Given the auxotrophic nature of pneumococci for certain amino acids, the Ami ABC transporter system, orchestrating oligopeptide uptake, becomes indispensable in host compartments lacking amino acids. The system comprises five exposed Oligopeptide Binding Proteins (OBPs) and four proteins building the ABC transporter channel. Crucially, SBPs determine the specificity of their respective transport systems, thereby governing the range of molecules capable of entering the cell. The five lipoproteins exhibit pairwise sequence identity of ~52–60% and share a very similar overall folding.

Consequently, the 1.8 Å-resolution open conformation of AliD was selected as a representative structure to describe the global architecture of OBPs in the Ami system. The obtained electron density map of the AliD structure, encompassing residues 28 to 652, presents an excellent quality all over the sequence. AliD adopts a bilobate structure characterized by three domains interconnected by short polypeptide chain segments serving as hinges. The two lobes enclose a deep cavity measuring ~16 Å in width and 45 Å in height, housing the peptide-binding pocket. Lobe 1 comprises Domain I (residues 29–63, 191–296, and 583–617) and Domain II (residues 64–190), while Lobe 2 consists solely Domain III (residues 297–582). The most striking feature of the AliD structure compared to OppA is the presence of an intriguing additional C-terminal 30-aa long α-helix (α19, spanning residues 622–652). This α-helix, which serves as distinctive hallmark of all the Ali proteins, establishes numerous hydrophobic and polar interactions with Domains I and II from Lobe 1, contributing significantly to the structural stability of the protein. The exposed surface of α19 is decorated with multiple basic residues, a conserved feature across all the OBPs in the Ami system that, besides its clear structural role, could help in proper orientation of the OBP on the membrane during oligopeptide binding. The ligand-bound and unbound forms of AliD retained the three-dimensional structures of the individual domains unaltered, as both conformations were related by a rigid-body rotation of ~20° of Lobe 1 (Domain III) relative to Lobe 2 (Domains I and III). AliD structure was solved by SAD technique.

> ASSDTKTYSSTFSGNPTTFNYLLDYYADNTAIITNLVDGLLENDNHGNLVPSLAEDWSVSSDGLTYTYKLRKDAKWFTADGEEYSPVKAQDFVTGIKYAVDNKSQAIDLIQNSIKGLNDYITGADSDFSKVGVKAIDDQTVEYTLARPEPYWNSKTTNSILFPVNEEFLNSKGKDFGTLSPDSILYSGPYLLKDFTSKSSIEYVKNPHYYDHDKVSIEHVKLAYFDGSDQELTIRNFESGAYSIAGVYPNSSNFAKTKEKYKDNIVYSLQDKTSWYFNFNVNRKAYNHTSKTTDEQKKSTETAVLNKNFRQAVNFALDRTAYSAQSNGEEAASKTLLNTLVPPTFVQVGDKTFGEVVASKLVNYGTEWSGINLADAQDAYFNKEKAQAKFAEAKKELTSQGVTFPIHLDVAVDQTSKNAVTGMNSVKQTLESVLGSDNIVIDVQQLSTDDFNNVAFLAPTAADRDYDFNFDGWVGDYQDPSTYLNPFNAEDGFYLKIFGLDAKEDKEKITSLGLDTYTKMLKDADRENKDVAKRYEKYAEAQAWMIDNSLIMSAMSSGGTASVTKVTPFTRGYSLVGIKGDGNNYKYMKLQKDTVTTKQFEEAKSKWEQESKKAIEKAQKEAEKHVK>LTCVTSKSIFGITTENCPDGQNLCFKRWQYISPRMYDFTRGCAATCPKAEYRDVINCCGTDKCNK[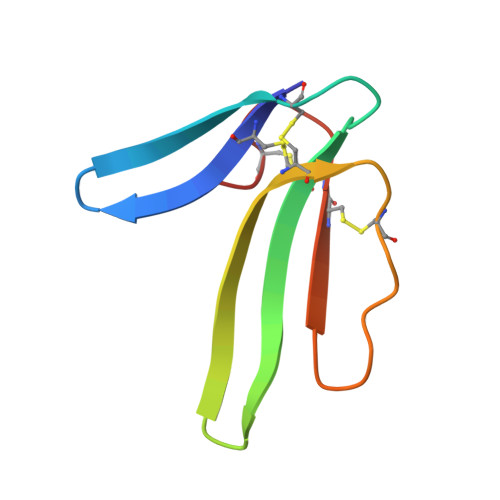3x]methyl 3-[4-[(4-bromophenyl)methyl]piperazin-1-yl]carbonyl-5-[(2-ethyl-2-methanoyl-butanoyl)amino]benzoate | C27 H32 Br N3 O5 | 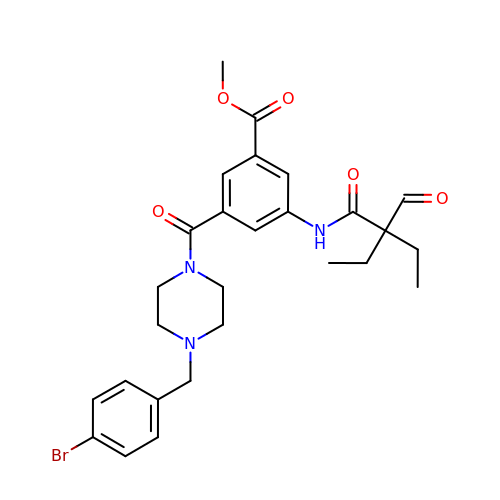DFOATAYHEDCOCM-UHFFFAOYSA-N> GSV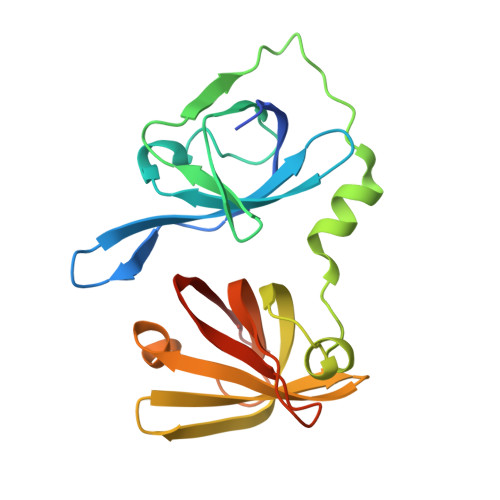DDSAQSDLKEVMVLNATESFVYEPKEQKKMFHATVATENEVFRVKVFNIDLKEKFTPKKIIAIANYVCRNGFLEVYPFTLVADVNADRNMEIPAGLIASASVTPKINQLCSQTKGSFVNGVFEVHKKNVRGEFTYYEIQDATGKMEVVVHGRLTTINCEEGDKLKLTCFELAPKSGNTGELRSVIHSHIKVIKTRKN>[6x]MPVAGSELPRRPLPPAAQERDAEPRPPHGELQYLGQIQHILRCGVRKDDRTGTGTLSVFGMQARYSLRDEFPLLTTKRVFWKGVLEELLWFIKGSTNAKELSSKGVKIWDANGSRDFLDSLGFSTREEGDLG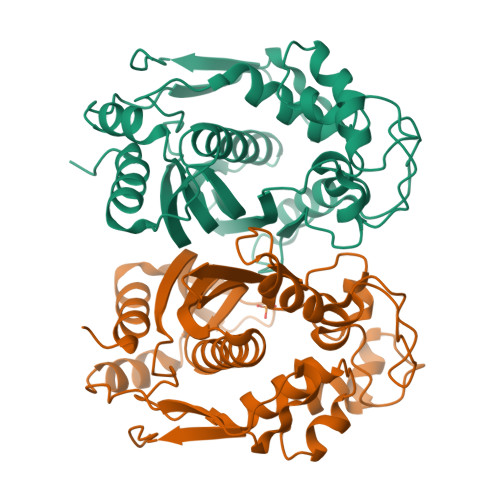PVYGFQWRHFGAEYRDMESDYSGQGVDQLQKVIDTIKTNPDDRRIIMCAWNPRDLPLMALPPCHALCQFYVVNSELSCQLYQRSGDMGLGVPFNIASYALLTYMIAHITGLKPGDFIHTLGDAHIYLNHIEPLKIQLQREPRPFPKLRILRKVEKIDDFKAEDFQIEGYNPHPTIKMEMAV>[3x]MDFLS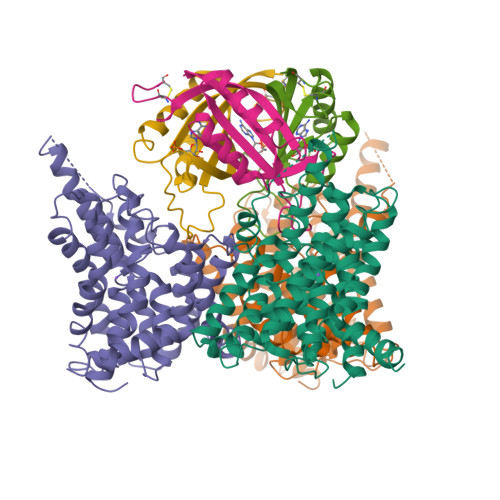NFLTDFVGQLQSPTLAFLIGGMVIAALGTQLVIPEAISTIIVFMLLTKIGLTGGMAIRNSNLTEMLLPVAFSVILGILIVFIARFTLAKLPNVRTVDALATGGLFGAVSGSTMAAALTTLEESKISYEAWAGALYPFMDIPALVTAIVVANIYLNKRKRKSAAASIEESFSKQPVAAGDYGDQTDYPRTRQEYLSQQEPEDNRVKIWPIIEESLQGPALSAMLLGLALGIFTKPESVYEGFYDPLFRGLLSILMLIMGMEAWSRIGELRKVAQWYVVYSLIAPIVHGFIAFGLGMIAHYATGFSLGGVVVLAVIAASSSDISGPPTLRAGIPSANPSAYIGSSTAIGTPIAIGVCIPLFIGLAQTLGAG;>MAKPANKLVIVTEKILLKKIAKIIDESGAKGYTVMNTGGKGSRNVRSSGQPNTSDIEANIKFEILTETREMAEEIADRVAVKYFNDYAGIIYICSAEVLYGHTFCGPEGC[3x]>GTQGKVIKCKAAIAWKTGSPLCIEEIEVSPPKACEVRIQVIATCVCHTDINATDPKKKALFPVVLGHECAGIVESVGPGVTNFKPGDKVIPFFAPQCKRCKLCLSPLTNLCGKLRNFKYPTIDQELMEDRTSRFTCKGRSIYHFMGVSSFSQYTVVSEANLARVDDEANLERVCLIGCGFSSGYGAAINTAKVTPGSTCAVFGLGCVGLSAIIGCKIAGASRIIAIDINGEKFPKAKALGATDCLNPRELDKPVQDVITELTAGGVDYSLDCAGTAQ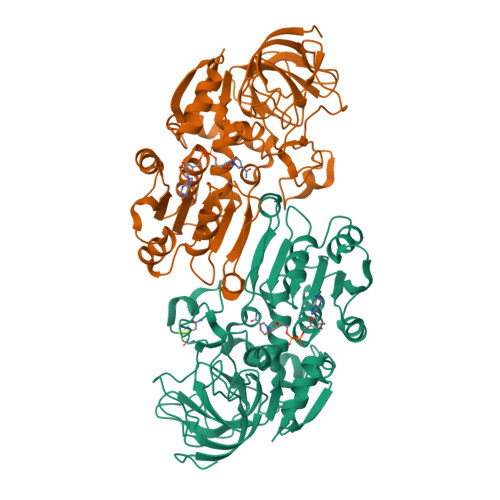TLKAAVDCTVLGWGSCTVVGAKVDEMTIPTVDVILGRSINGTFFGGWKSVDSVPNLVSDYKNKKFDLDLLVTHALPFESINDAIDLMKEGKSIRTILTF[2x]Bilirubin is conjugated in hepatocytes and excreted to bile duct via the ATP-binding cassette transporter ABCC2, dysfunction of which would lead to Dubin-Johnson syndrome. ABCC2 is a 180 kDa full transporter of 1545 residues that structurally consists of two half modules, which are predicted to be the transmembrane domain (TMD) and a cytoplasmic nucleotide-binding domain (NBD), respectively. Notably, ABCC2 also has an extra N-terminal TMD0, which exists mainly in ABCC family and was suggested to participate in the subcellular localization. Here we determine the structures of ABCC2 in the apo, substrate-bound and ATP/ADP-bound forms using the cryo-electron microscopy, exhibiting a full transporter with a regulatory (R) domain inserted between the two half modules.

The apo-form structure of ABCC2 shows an inward-facing (IF) conformation. In the translocation cavity, we found an extra density that could be fitted by the N- and M-segment of the R domain, in which only the side chains of the M-segment can be well fitted due to a relatively higher local resolution. The M-segment is folded into a short helix and a loop, occupying the translocation cavity, whereas the densities of the C-segment are untraceable in the map. The M-segment of the R domain is fixed in translocation cavity via abundant hydrogen bonds and salt bridges with the residues from TMD1 and TMD2. Specifically, Glu892 from the loop of the M-segment forms a hydrogen bond with Tyr381 from TMD1. In addition, Glu893 forms a hydrogen bond with Asn1204 and two salt bridges with Arg1205 and Arg1257 of TMD2, respectively. Arg904 from the helix forms a salt bridge with Glu1261 of TMD2. To investigate the function of the M-segment that binds to the translocation cavity, we generated the variants E892Q and E893Q for ATPases activity assays. Interestingly, both variants displayed a significant increase of ATPase activity compared to the wild type. We further performed the transport activity assays using radioisotope-labeled substrate E217βG and found that E892Q and E893Q also exhibited a significant increase of transport activity. Thus, these results indicated that the R domain binding to the translocation cavity functions as an auto-inhibitor of ABCC2.

> MLEKFCNSTFWNSSFLDSPEADLPLCFEQTVLVWIPLGYLWLLAPWQLLHVYKSRTKRSSTTKLYLAKQVFVGFLLILAAIELALVLTEDSGQATVPAVRYTNPSLYLGTWLLVLLIQYSRQWCVQKNSWFLSLFWILSILCGTFQFQTLIRTLLQGDNSNLAYSCLFFISYGFQILILIFSAFSENNESSNNPSSIASFLSSITYSWYDSIILKGYKRPLTLEDVWEVDEEMKTKTLVSKFETHMKRELQKARRALQRRQEKSSQQNSGARLPGLNKNQSQSQDALVLEDVEKKKKKSGTKKDVPKSWLMKALFKTFYMVLLKSFLLKLVNDIFTFVSPQLLKLLISFASDRDTYLWIGYLCAILLFTAALIQSFCLQCYFQLCFKLGVKVRTAIMASVYKKALTLSNLARKEYTVGETVNLMSVDAQKLMDVTNFMHMLWSSVLQIVLSIFFLWRELGPSVLAGVGVMVLVIPINAILSTKSKTIQVKNMKNKDKRLKIMNEILSGIKILKYFAWEPSFRDQVQNLRKKELKNLLAFSQLQCVVIFVFQLTPVLVSVVTFSVYVLVDSNNILDAQKAFTSITLFNILRFPLSMLPMMISSMLQASVSTERLEKYLGGDDLDTSAIRHDCNFDKAMQFSEASFTWEHDSEATVRDVNLDIMAGQLVAVIGPVGSGKSSLISAMLGEMENVHGHITIKGTTAYVPQQSWIQNGTIKDNILFGTEFNEKRYQQVLEACALLPDLEMLPGGDLAEIGEKGINLSGGQKQRISLARATYQNLDIYLLDDPLSAVDAHVGKHIFNKVLGPNGLLKGKTRLLVTHSMHFLPQVDEIVVLGNGTIVEKGSYSALLAKKGEFAKNLKTFLRHTGPEEEATVHDGSEEEDDDYGLISSVEEIPEDAASITMRRENSFRRTLSRSSRSNGRHLKSLRNSLKTRNVNSLKEDEELVKGQKLIKKEFIETGKVKFSIYLEYLQAIGLFSIFFIILAFVMNSVAFIGSNLWLSAWTSDSKIFNSTDYPASQRDMRVGVYGALGLAQGIFVFIAHFWSAFGFVHASNILHKQLLNNILRAPMRFFDTTPTGRIVNRFAGDISTVDDTLPQSLRSWITCFLGIISTLVMICMATPVFTIIVIPLGIIYVSVQMFYVSTSRQLRRLDSVTRSPIYSHFSETVSGLPVIRAFEHQQRFLKHNEVRIDTNQKCVFSWITSNRWLAIRLELVGNLTVFFSALMMVIYRDTLSGDTVGFVLSNALNITQTLNWLVRMTSEIETNIVAVERITEYTKVENEAPWVTDKRPPPDWPSKGKIQFNNYQVRYRPELDLVLRGITCDIGSMEKIGVVGRTGAGKSSLTNCLFRILEAAGGQIIIDGVDIASIGLHDLREKLTIIPQDPILFSGSLRMNLDPFNNYSDEEIWKALELAHLKSFVASLQLGLSHEVTEAGGNLSIGQRQLLCLGRALLRKSKILVLDEATAAVDLETDNLIQTTIQNEFAHCTVITIAHRLHTIMDSDKVMVLDNGKIIECGSPEELLQIPGPFYFMAKEAGIENVNSTKFLEDYKDDDDKVEHHHHHHHH>NVAELKKSFNRHLHFTLVKDRNVATTRDYYFALAHTVRDHLVGRWIRTQQHYYDKCPKRVYYLSLEFYMGRTLQNTMINLGLQNACDEAIYQLGLDIEELEEIEEDAGLGNGGLGRLAACFLDSMATLGLAAYGYGIRYEYGIFNQKIRDGWQVEEADDWLRYGNPWEKSRPEFMLPVHFYGKVEHTNTGTKWIDTQVVLALPYDTPVPGYMNNTVNTMRLWSARAPNDFNLRDFNVGDYIQAVLDRNLAENISRVLYPNDNFFEGKELRLKQEYFVVAATLQDIIRRFKASKFGSTRGAGTVFDAFPDQVAIQLNDTHPALAIPELMRIFVDIEKLPWSKAWELTQKTFAYTNHTVLPEALERWPVDLVEKLLPRHLEIIYEINQKHLDRIVALFPKDVDRLRRMSLIEEEGSKRINMAHLCIVGSHAVNGVAKIHSDIVKTKVFKDFSELEPDKFQNKTNGITPRRWLLLCNPGLAELIAEKIGEDYVKDLSQLTKLHSFLGDDVFLRELAKVKQENKLKFSQFLETEYKVKINPSSMFDVQVKRIHEYKRQLLNCLHVITMYNRIKKDPKKLFVPRTVIIGGKAAPGYHMAKMIIKLITSVADVVNNDPMVGSKLKVIFLENYRVSLAEKVIPATDLSEQISTAGTEASGTGNMKFMLNGALTIGTMDGANVEMAEEAGEENLFIFGMRIDDVAALDKKGYEAKEYYEALPELKLVIDQIDNGFFSPKQPDLFKDII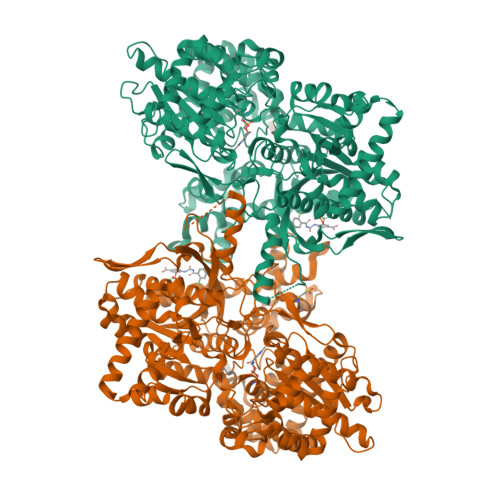NMLFYHDRFKVFADYEAYVKCQDKVSQLYMNPKAWNTMVLKNIAASGKFSSDRTIKEYAQNIWNVEPSD[2x]>[4x]KNVTLTIRLLMHGKEV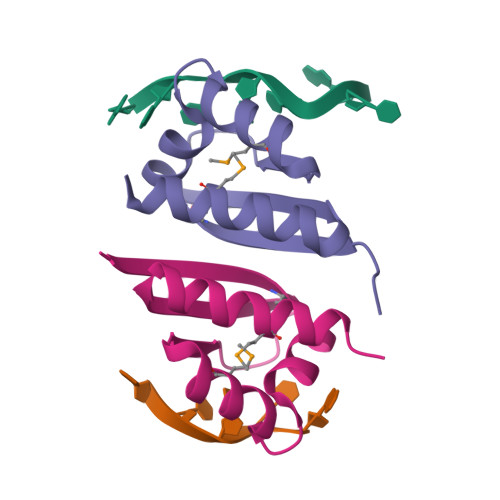GSIIGKKGESVKKMREESGARINISEGNCPERIITLAGPTNAIFKAFAMIIDKLEED The organometallic nickel-pincer nucleotide (NPN) cofactor is composed of a nickel ion pincered by two sulfur and one carbon atoms from a pyridinium 3,5-dithiocarboxylate mononucleotide (P2TMN). Notably, although most LarAHs possess two catalytic histidine residues that are essential for the PCHT mechanism, the second histidine residue (His174 in LarALp) in a small fraction of LarAHs is substituted by other amino acids, often an asparagine which cannot function as a general acid/base in catalysis. In this study, we characterized two members of a newly identified LarA subfamily that lacks one of the catalytic histidine residues conserved in other LarAHs. From the structural data, combined with MS and spectroscopic analysis, as well as genomic context analysis, our findings revealed (1) a unique octameric assembly which is unprecedented among other known LarAHs; (2) a distinct set of active site residues, including the asparagine side chain substitution for the missing histidyl group, suggesting recognition and processing of non-canonical LarA substrates; and (3) genomic and structural evidence hypothetically linking these LarAHs to carbohydrate metabolism.

To generate a LarAH in this subfamily in the holo state, we cloned the gene for a homolog of LarABw from S. plurextorum, a pathogen of swine, which shares 72% identical residues with LarABw, and we co-expressed the C-terminal strep-tagged protein with LarB/C/D/E in L. lactis. Importantly, the purified protein exhibited a yellowbrown color, which is consistent with the holo state of LarAHs. Like LarABw, LarASp also assembles as an octamer that is a tetrameric dimer, and the monomeric protein has a putative active site between the N- and C-domains. Arg431 (equivalent to Arg434 in LarABw) forms multiple hydrogen bonds with the same set of residues from the other protomer as in LarABw at the dimerization interface, suggesting that the tail-to-tail dimer is common in this LarA subfamily whereas octamerization may not be so prevalent since the residues at the interface between the neighboring dimers are not conserved. At the active site, a continuous density matches the NPN cofactor. As this density is connected to the side chain of Lys195, the NPN cofactor forms a covalent linkage through a thioamide bond to the enzyme. Like in LarALp and LarAIp, the nickel atom in the NPN cofactor is coordinated to the C4 atom of the pyridinium ring, two sulfur atoms, and the imidazole side chain of His211 in a square-planar coordination. Over the NPN cofactor, we noticed electron density in close proximity to the conserved His115, His306, Tyr307, and His401, occupying a position corresponding to the substrate binding sites of other LarAHs.

>[8x]MKIDFEYGHGTMTADLPDTTDIFIPGETVADPECLPEDQIEAATLDSIRNPLGMPPLTELAKPGSKVTIVFPDRVKGGEQATAHRKVSIKLILQELYSVGVKKEDILLICSNGLHRKNTEKEILGVLGPDLYHQFAPTGQIINHDSEDYEHLVDLGKTKQGDPVIMNKYVYESDVAILIGHTQGNPYGGYSGGYKHCSTGITHWKSIASHHVPKVMHRKDFVPVNNNSLMRHKFDEIGMHMEEKMGKKFFCCDAVLDTKSRQIEINSGAADEVQKKAWKLGNARTYVPFAEKKYDIIVFGMPQFFHYGDGMGTNPIMLMQALSAQVIRHKRIMSDNCVFICASTCNGYFNESLWPYLPELYDLFQKEGNTLVDLNQYGEYFATNEEYIRKYRYAHAFHPFHGFSMISCAHLAEKHTAAIYLVGAEKPGYARGMGLKTRATFEEALEDAKKKFVGQEPNILALPKAFKTAAVHLMMKNDLPPMTPRYEENHWSHPQFEK> LTAKKRPSVVYLHNAECTGCSESVLRTVDPYVDELILDVISMDYHETLMAGAGHAVEEALHEAIKGDFVCVIEGGIPMGDGGYWGKVGGRNMYDICAEVAPKAKAVIAIGTCATYGGVQAAK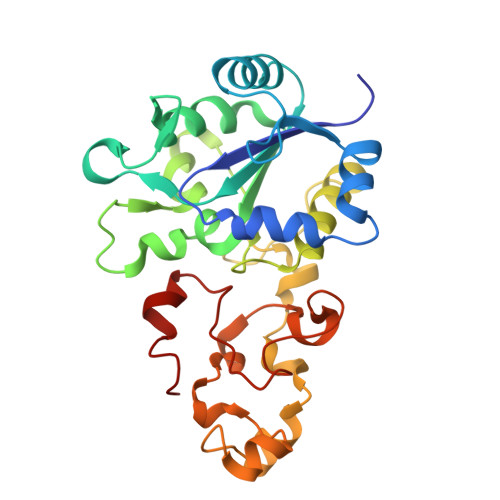PNPTGTVGVNEALGKLGVKAINIAGCPPNPMNFVGTVVHLLTKGMPELDKQGRPVMFFGETVHDNCPRLKHFEAGEFATSFGSPEAKKGYCLYELGCKGPDTYNNCPKQLFNQVNWPVQAGHPCIACSEPNFWDLYSPFYSA> LMSGQRGLDLHVLSAPCRPCSDTEVLLAICTSDFVVRGFIEDVTHVPEQQVSVIYLRVNRLHRQKSRVFQPAPEDSGHWLGHVTTLLQCGVRPGHGEFLFTGHVHFGEAQLGCAPRFSDFQRMYRKAEEMGI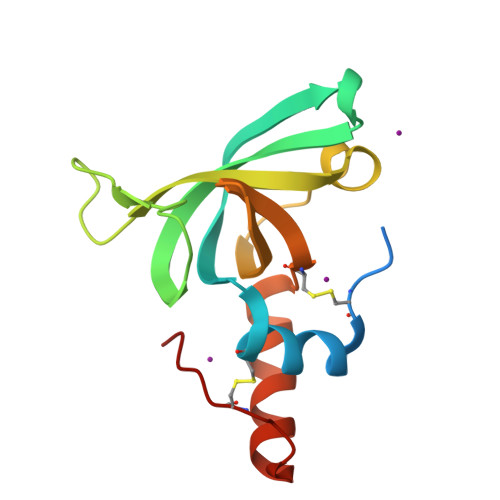NPCEINME>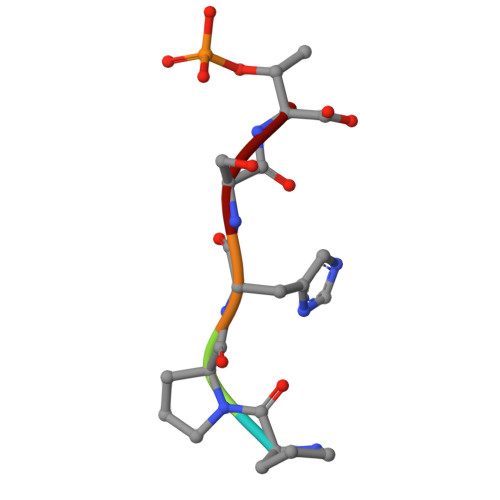 PPHST> GRLWLPNTPDASDPQRGRLAPPGELNLTTASVPMLRWYAERFCFVLVTTAEFPRDPGQLLYIPKTYLLGRPRNASLPELPEAGPTSRPPAEVTQLKG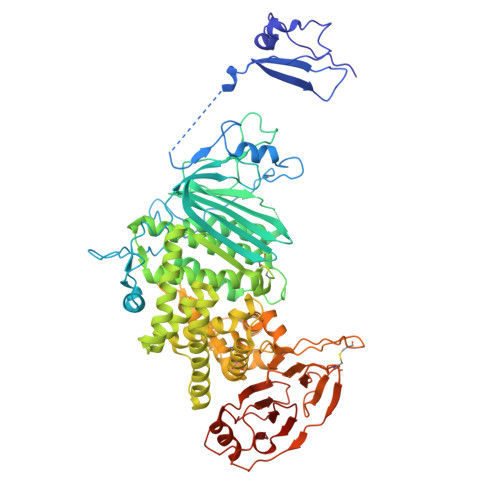LSHNPGASALLRSRAWVTFAAAPDREGLTFPRGDDGATERHPDGRRNAPPPGPPAGTPRHPTTNLSIAHLHNASVTWLAARGLLRTPGRYVYLSPSASTWPVGVWTTGGLAFGCDAALVRARYGKGFMGLVISMRDSPPAEIIVVPADKTLARVGNPTDENAPAVLPGPPAGPRYRVFVLGAPTPADNGSALDALRRVAGYPEESTNYAQYMSRAYAEFLGEDPGSGTDARPSLFWRLAGLLASSGFAFVNAAHAHDAIRLSDLLGFLAHSRVLAGLAARGAAGCAADSVFLNVSVLDPAARLRLEARLGHLVAAILEREQSLVAHALGYQLAFVLDSPAAYGAVAPSAARLIDALYAEFLGGRALTAPMVRRALFYATAVLRAPFLAGAPSAEQRERARRGLLITTALCTSDVAAATHADLRAALARTDHQKNLFWLPDHFSPCAASLRFDLAEGGFILDALAMATRSDIPADVMAQQTRGVASVLTRWAHYNALIRAFVPEATHQCSGPSHNAEPRILVPITHNASYVVTHTPLPRGIGYKLTGVDVRRPLFITYLTATCEGHAREIEPKRLVRTENRRDLGLVGAVFLRYTPAGEVMSVLLVDTDATQQQLAQGPVAGTPNVFSSDVPSVALLLFPNGTVIHLLAFDTLPIATIAPHHHHHH>[2x]GDSVEKIVLELSGLSCHHCVARVKKALEEAGAKVE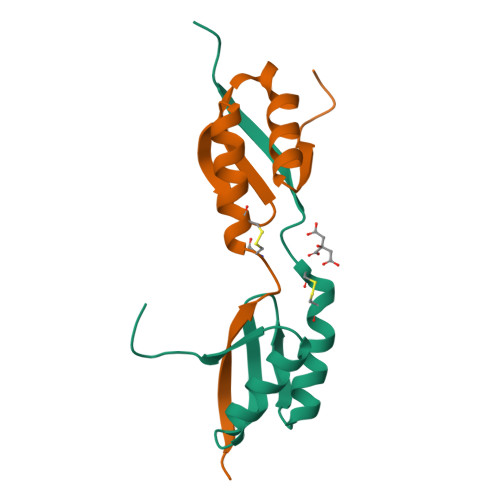KVDLNEAVVAGNKEDVDKYIKAVEAAGYQAKLRSSAWS> MFFSQVLRSSARAAPIKRYTGGRIGESWVI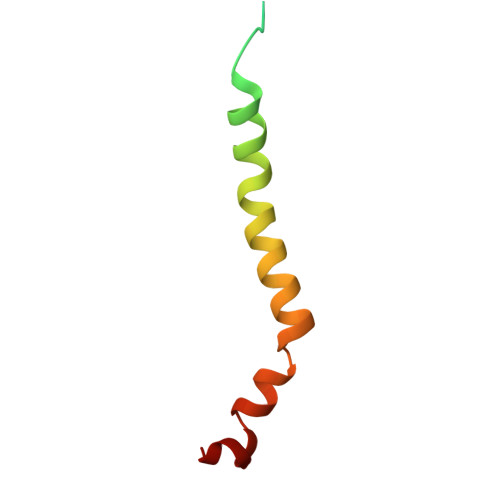TEGRRLIPEIFQWSAVLSVCLGWPGAVYFFSKARKA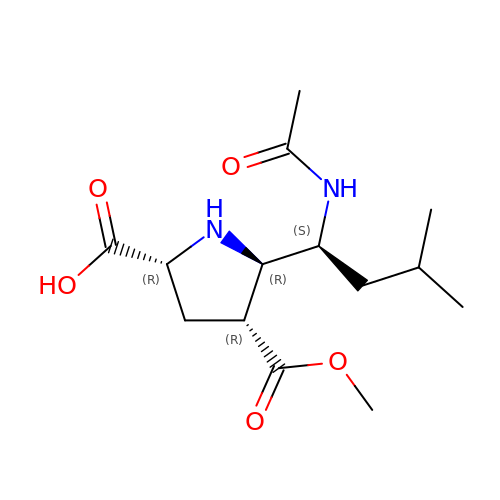5-[1-(ACETYLAMINO)-3-METHYLBUTYL]-4-(METHOXYCARBONYL)PROLINE | C14 H24 N2 O5 | OXAVBPLKPVSWSQ-WRWGMCAJSA-N>[7x]MKTLIVVDMQNDFISPLGSLTVPKGEELINPISDLMQDADRDWHRIVVTRDWHPSRHISFAKNHKDKEPYSTYTYHSPRPGDDSTQEGILWPVHCVKNTWGSQLVDQIMDQVVTKHIKIVD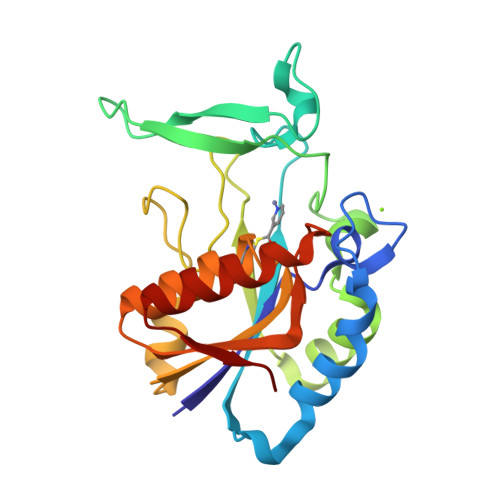KGFLTDREYYSAFHDIWNFHKTDMNKYLEKHHTDEVYIVGVALEYCVKATAISAAELGYKTTVLLDYTRPISDDPEVINKVKEELKAHNINVVDK> PGSSPPTCRSKCGKCQP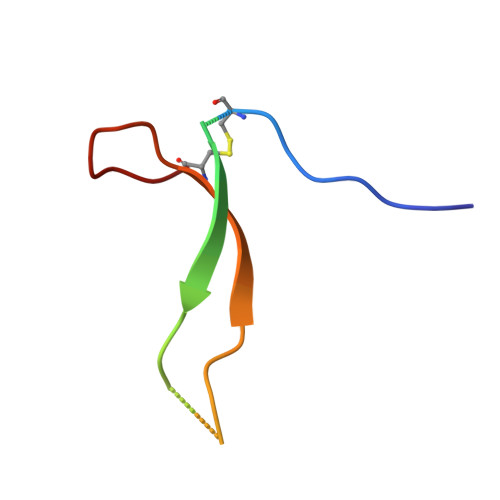CKPVHVPIQPGLSMPLEYYPEAWRCKCGNKLFMP>SDAHHAHKGLNYGSFTKEHVLLTPKGYREWVFIGASVTPNELNDDKAAFPEFHNVYIDPTSWGHWK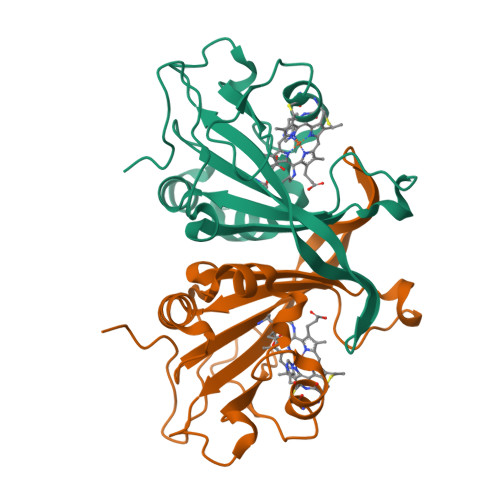KTGEFRDGTVIVKELAGVGSKASPSGNGYFPGEFNGIQAMVKDSKRYPERPGNWAFFGFESYEAKQGIIQTDETCAACHKEHAAHDMVFTQFYPVLRAGKPSK[4x]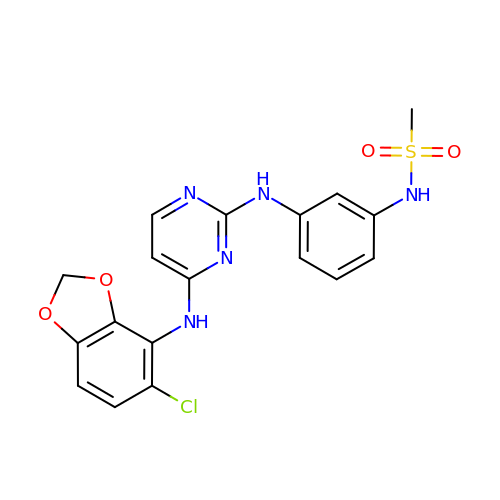N-[3-[[4-[(5-CHLORO-1,3-BENZODIOXOL-4-YL)AMINO]PYRIMIDIN-2-YL]AMINO]PHENYL]METHANESULFONAMIDE | C18 H16 Cl N5 O4 S | KQGTYXRWSIBDOZ-UHFFFAOYSA-N(2S)-1-[(2-fluorobenzyl)oxy]-3-(pyrrolidin-1-yl)propan-2-ol 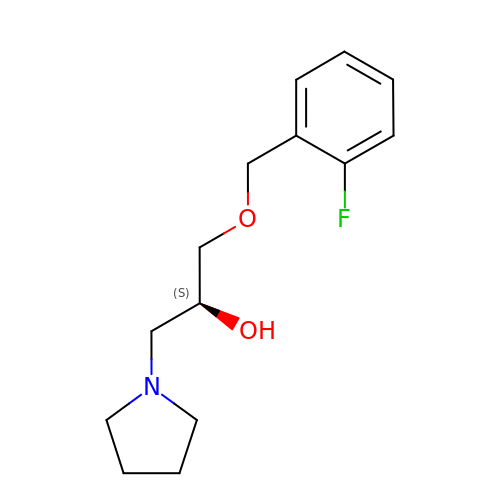| C14 H20 F N O2 | HWPXULNASVXWSB-ZDUSSCGKSA-N>MIYPDEAMLYAPVEWHDCSEGFEDIRYEKSTDGIAKITINRPQVRNAFRPLTVKEMIQALADARYDDNIGVIILTGAGDKAFCSGGDQKVRGDYGGYKDDSGVHHLNVLDFQRQIRTCPKPVVAMVAGYSIGGGHVLHMMCDLTIAADNAIFG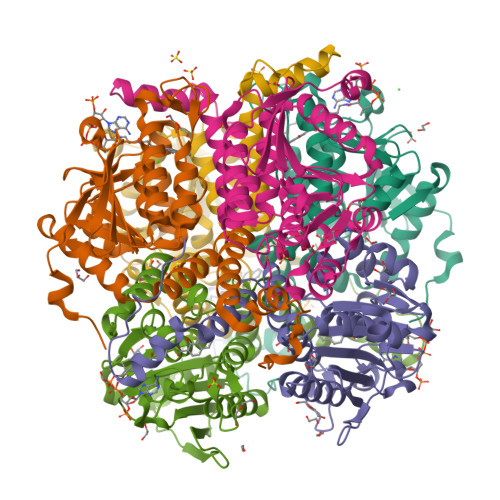QTGPKVGSFDGGWGASYMARIVGQKKAREIWFLCRQYDAKQALDMGLVNTVVPLADLEKETVRWCREMLQNSPMALRCLKAALNADCDGQAGLQELAGNATMLFYMTEEGQEGRNAFNQKRQPDFSKFKRNP[12x]>[3x]RVSLNFKDPEAVRALTCTLLREDFGLS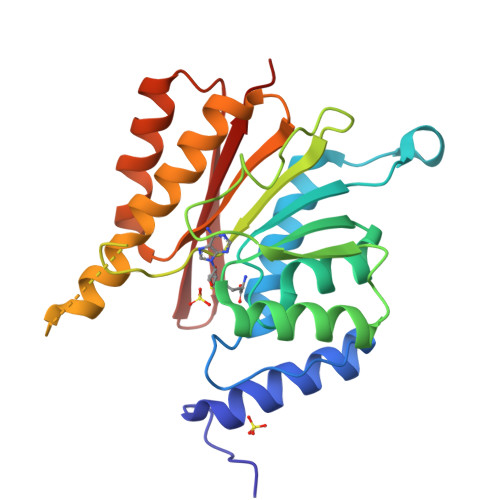IDIPLERLIPTVPLRLNYIHWVEDLIGHQDSDKSTLRRGIDIGTGASCIYPLLGATLNGWYFLATEVDDMCFNYAKKNVEQNNLSDLIKVVKVPQKTLLMDALKEESEIIYDFCMCNPPFFANQLEAKGVNSRNPRRPPPSSVNTGGITEIMAEGGELEFVKRIIHDSLQLKKRLRWYSCMLGKKCSLAPLKEELRIQGVPKVTYTEFCQGRTMRWALAWSFYD GORK is a shaker-like potassium channel in plants that contains ankyrin (ANK) repeats. GORK, also known as guard cell outward rectifying K+ channel, is the only outward-rectifying potassium channel in guard cells. In contrast, GORK activation causes potassium efflux, reducing guard cell turgor and volume and in turn stomatal closure. Each protomer has an N-terminal transmembrane domain (TMD, residues 58–313, containing helices S1–S6), followed by three cytoplasmic domains: the C-linker (residues 314–365), cyclic nucleotide-binding domain homolog (CNBDH) (residues 366–510), and ANK (residues 511–724).

Tetrameric reconstructions of AtGORK were obtained in two conformational states at resolutions of 3.4 Å (AtGORKFL1) and 4.3 Å (AtGORKFL2), allowing de novo modeling of 662 of 820 amino acids (residues 58–720) for each protomer, while the remaining regions were not resolved due to their intrinsic flexibility. The full-length AtGORKFL forms a tetramer with elongated cytoplasmic regulatory domains, with its architecture showing a symmetry reduction from four-fold (C4) to two-fold (C2). Notably, the symmetry in the TMD portion adopts a typical four-fold (C4), but reduces to a two-fold (C2) in their following cytoplasmic domains, thus leading to a deformation within the tetrameric channel. Remarkably, ANK repeats from two neighboring protomers form a stable dimer through specific interactions mediated by their protruding loops, creating a buried area of ~1,500 Å2. As a result of ANK dimerization, positional deviations and conformational changes are induced in the adjacent CNBDH and C-linker, leading to a reduction in symmetry within the tetrameric channel. This reduction affects the communication and coupling between cytoplasmic domains and transmembrane helices, ultimately maintaining GORK in an autoinhibited, preactivation state. Due to the reduced symmetry within the tetramer, the C-linkers exhibits distinct conformations between adjacent protomers, either “flat” or “kinked”. Consequently, the C-linker in AtGORK deviates from C4 symmetry, and the presence of the “flat” conformation disrupts the formation of a C4 symmetrical gating ring, leading to decoupling between the transmembrane helices and the cytoplasmic domains, ultimately affecting channel gating. In contrast, the TMD of full-length AtGORKFL1 displays quasi-C4 symmetry (essentially C2 symmetry), with subtle yet distinct differences between protomers A/C and B/D at the N-terminal end of helix S5, yielding an RMSD of approximately 0.75 Å/256 superimposed Cα. Analysis using the HOLE suggests that the AtGORK adopts a closed conformation.

>[4x]IHPKNRWYKAWEMFILVWAIYSSLFTPMEFGFFRGLPERLFVLDIVGQIAFLVDIVLQFFVAYRDTQTYRTVYKPTRIAFRYLKSHFLMDFIGCFPWDLIYKASGKHELVRYLLWIRLFRVRKVVEFFQRLEKDTRINYLFTRILKLLFVEVYCTHTAACIFYYLATTLPPENEGYTWIGSLKLGDYSYENFREIDLWKRYTTALYFAIVTMATVGYGDIHAVNLREMIFVMIYVSFDMVLGAYLIGNITALIVKGSNTERFRDKMNDLISFMNRKKLGRDLRSQITGHVRLQYDSHYTDTVMLQDIPASIRAKIAQLLYLPYIKKVPLFKGCSTEFINQIVIRLHEEYFLPGEVITEQGNVVDHLYFVCEGLLEALVTKTDGSEESVTLLGPHTSFGDISIICNISQPFTVRVCELCHLLRLDKQSFSNILEIYFHDGRTILNNIMEEKESNDRIKKLESDIVIHIGKQEAELALKVNSAAFQGDFYQLKSLIRSGADPNKTDYDGRSPLHLAACRGYEDITLFLIQEGVDVNLKDKFGHTPLFEAVKAGQEGVIGLLVKEGASFNLEDSGNFLCTTVAKGDSDFLKRLLSSGMNPNSEDYDHRTPLHVAASEGLFLMAKMLVEAGASVISKDRWGNSPLDEARLCGNKKLIKLLEDVKNAQSSIYPSSLRELQEERIERRKCTVFPFHPQEAKEERSRKHGVVVWIPSNLEKLIVTAAKELGLSDGASFVLLSEDQGRITDIDMISDGHKLYMISDTTDQT Focal Adhesion Kinase (FAK) is a non-receptor tyrosine kinase that regulates signals involved in cell proliferation, migration and survival. FAK activation is initiated by breaking an intramolecular autoinhibitory interaction between the N-terminal FERM (4.1, ezrin, radixin, moesin homology) and kinase domains. All compounds exhibit a common 5-chloro-2-ortho-methoxyanilino-4-anilinopyrimidine core structure, which binds in a nearly identical manner to the hinge region of the FAK kinase.

In contrast, AZW592, which has a sulfamoyl group at the corresponding position, makes no significant interactions with the activation loop, but several water molecules fill the space between the compound and the activation loop. The activation loop in the AZW592 bound FAK kinase follows a non-helical path similar to the one observed in autoinhibited FAK. This allows the gatekeeper residue Met499 to rotate its sidechain towards AZW592 and it makes van der Waals contact with the chlorine atom on the pyrimidine ring. The morpholine (TAE226), methylpiperazine (TAF089), dipiperidine (TAF672) or methylaminopyrrolidine (AZW592) moieties in para position to the amine groups of the aniline rings make almost no protein contacts, consistent with their incorporation for improved pharmacokinetic properties of the respective compounds. Additionally, an analog of TAE226 that fails to induce the helical DFG conformation displays a 3-fold lower potency. We evaluated the potencies of the FAK inhibitors by determining dose-response kinase inhibition curves and deriving IC50 values. As apparent from Table 2, TAE226 and TAF089 exhibit approximately 3-fold higher potencies than AZW592.

> STRDYEIQRERIELGRCIGEGQFGDVHQGIYMSPENPAMAVAIKTCKNCTSDSVREKFLQEALTMRQFDHPHIVKLIGVITENPVWIIMELCTLGELRSFLQVRKYSLDLASLILYAYQLSTALAYLESKRFVHRDIAARNVLVSSNDCVKLGDFGLSRYMEDSTYYKASKGKLPIKWMAPESINFRRFTSASDVWMFGVCMWEILMHGVKPFQGVKNNDVIGRIENGERLPMPPNCPPTLYSLMTKCWAYDPSRRPRFTELKAQLSTILEEEKLQ>MPELPEVETTLRGIAPHIEGKTVEAVVLRQLKLRWQINPDLGEILSGRQVLSCGRRAKYLLIRFQTGVLLIHLGMSGSLRIFTPSDGRIGRPDRHDHVDIVFSDGTVMRYRDPRKFGAILWYEGIEEHHPLLEKLGPEPLSEAFCADYLYARLKAQKRAVK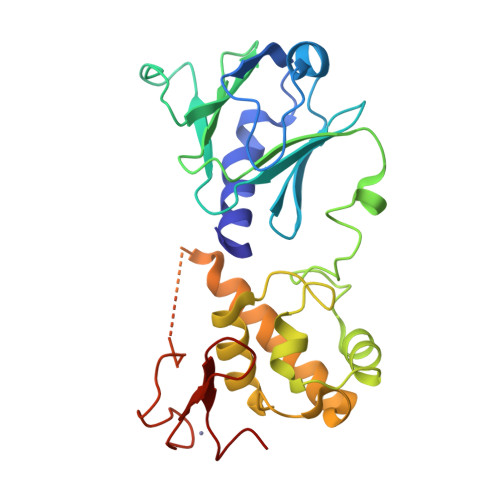LALMDNAVVVGVGNIYANESLFRAGISPHRPANRLKKKECALLVETVKAVLQRAIETGGSTLRDFVDSDGKSGYFQQEYTVYGRHNQPCPRCGGLVVKETLGQRGTFYCPNCQK[2x]> EGFIDDSTLTGGIYYWQRERDRKDVTDGDKYKTNLSHSTWNANLDF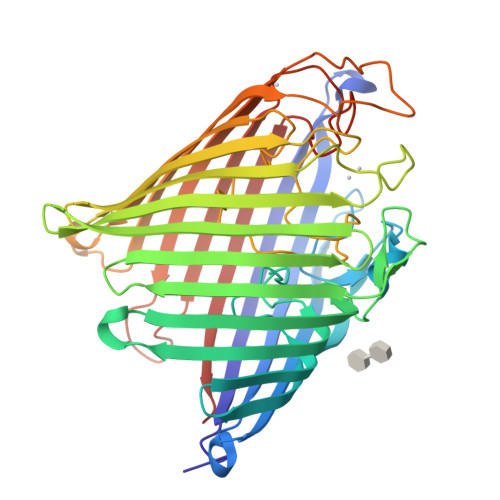QSGYAADMFGLDIAAFTAIEMAENGDSSHPNEIAFSKSNKAYDEDWSGDKSGISLYKAAAKFKYGPVWARAGYIQPTGQTLLAPHWSFMPGTYQGAEAGANFDYGDAGALSFSYMWTNEYKAPWHLEMDEFYQNDKTTKVDYLHSFGAKYDFKNNFVLEAAFGQAEGYIDQYFAKASYKFDIAGSPLTTSYQFYGTRDKVDDRSVNDLYDGTAWLQALTFGYRAADVVDLRLEGTWVKADGQQGYFLQRMTPTYASSNGRLDIWWDNRSDFNANGEKAVFFGAMYDLKNWNLPGFAIGASYVYAWDAKPATWQSNPDAYYDKNRTIEESAYSLDAVYTIQDGRAKGTMFKLHFTEYDNHSDIPSWGGGYGNIFQDERDVKFMVIAPFTIFHHHHHH> MSTPNSYDDEELEELLRR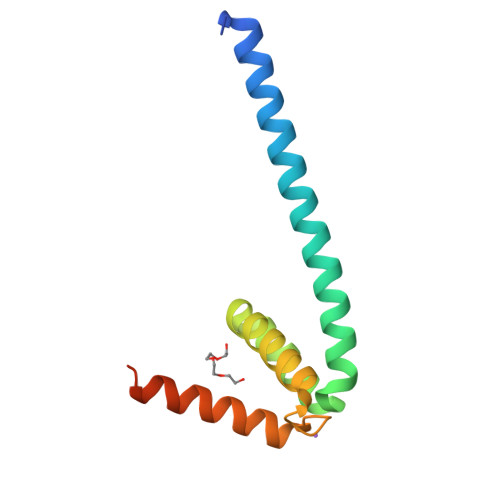KAAQEQKRIEEERKRKAELESQKESILRVILTPEARQRLTNIKLVKPEFAESLENQLIALAQSGRIKIPITDEELKQILEQISQQNRRDFKIQIRERGWK>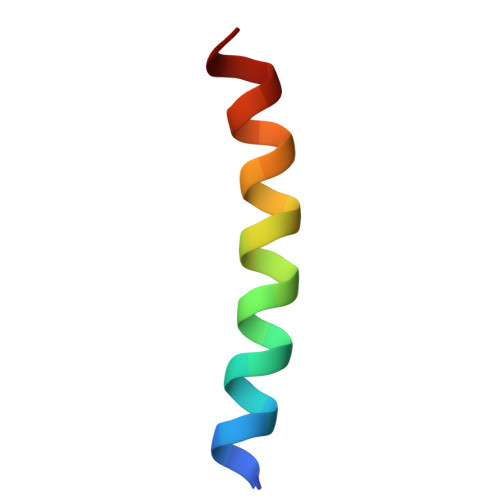 SAQQELKQRQRAEIYALNRVMTELEQ Human CEACAM1 (hCEACAM1) is a single pass type I transmembrane protein expressed as 12 alternatively spliced isoforms that all contain an N-terminal V set fold of the immunoglobulin superfamily (IgV) ectodomain followed by up to three type 2 constant immunoglobulin (IgC2) ectodomains (A1, B, A2), a transmembrane sequence, and a signaling cytoplasmic domain. CEACAM1 function is triggered by intercellular or trans binding of the IgV domain, resulting in higher order surface CEACAM1 oligomerization and subsequent intracellular signal transduction. In contrast to other immunoreceptors such as the T cell inhibitory and mucin domain-containing protein 3 (TIM-3), programmed cell death protein 1 (PD-1), and programmed death-ligand 1 (PD-L1), CEACAM1 serves as its own primary ligand, owing to high affinity homophilic interactions of its unique IgV domain, as well as an important microbial receptor. The displaced CC′ loop forms a cleft with the FG loop that exposes the key residues F29, S32, Y34, V39, G41, Q44, Q89, I91, N97, and E99 critical in mediating homophilic CEACAM1 interactions.

Another defining feature of the GFCC′ interface in the hCEACAM1 WT homodimer is the important contribution of N97 in mediating a critical hydrogen bond network comprising seven hydrogen bond interactions. In the N97A mutant crystal, we observed two monomeric N97A molecules [(a), (b)] in the asymmetric unit devoid of any GFCC′-mediated interactions despite high concentration (>800 μM) and global similarity in secondary structure of both N97A molecules (a) and (b) compared to hCEACAM1 WT (RMSD of 0.4 Å over 638 atoms and 0.6 Å over 628 atoms, respectively). In fact, only two residues participated in hydrogen bond interactions less than 3.5 Å apart between two molecules of N97A in the static crystal structure: Q26 of molecule (a) and I67 of molecule (b). Thus, the hCEACAM1 IgV N97A crystal structure highlighted the critical properties of an asymmetric hydrogen bond network crucial towards mediating hCEACAM1 IgV dimerization. The downfield G41 peak (indicator of an intermolecular hydrogen bond in the WT homodimer) was absent in the 15N-HSQC spectrum of N97A mutant, confirming a global conformation transition from a dimer to monomer state. The residues that shifted the most followed a distribution pattern similar to the chemical shift differences observed between WT and N97A mutant proteins at the GFCC′ face, consistent with the notion that the N97A protein resides in a rapid monomer–dimer dynamic equilibrium in the fast-to-intermediate exchange regime on the NMR timescale. Fitting the peak trajectories of residues Q44 and A49 provided a rough estimate of over 1 mM affinity (dissociation constant KD) for the hCEACAM1 N97A homodimer, consistent with the previous studies. While the crystal structure of the N97A mutant showed the lowest B factor value of 16 Å2, a closer examination revealed higher B factor profiles of the CC′, EF, and FG loop residues.

>QLTTESMPFNVAEGKEVLLLVHNLPQQLFGYSWYKGERVDGNRQIVGYAIGTQQATPGPANSGRETIYPNASLLIQNVTQNDTGFYTLQVIKSDLVAEEATGQFHVY[2x]>SNKCDVVVVGGGISGMAAAKLLHDSGLNVVVLEARDRVGGRTYTLRNQKVKYVDLGGSYVGPTQNRILRLAKELGLETYKVNEVERLIHHVKGKSYPFRGPFPPVWNPITYLDHNNFWRTMDDMGREIPSDAPWKAPLAEEWDNMTMKELLDKLCWTESAKQLATLFVNLCVTAETHEVSALWFLWYVKQCGGTTRIASTTNGGQERKFVGGSGQVSERIMDLLGDRVKLERPVIYIDQTRENVLVETLNHEMYEAKYVISAIPPTLGMKIHFNPPLPMMRNQMITRVPLGSVIKCIVYYKEPFWRKKDYCGTMIIDGEEAPVAATLDDTKPEGNYAAIMGFILAHKARKLARLTKEERLKKLCELYAKVLGSLEALEPVHYEEKNWCEEQYSGGCYTTYFPPGILTQYGRVLRQPVDRIYFAGTETATHWSGYMEGAVEAGERAAREILHAMGKIPEDEIWQSEPESVDVPAQPITTTFLERHLPSVPGLLRLI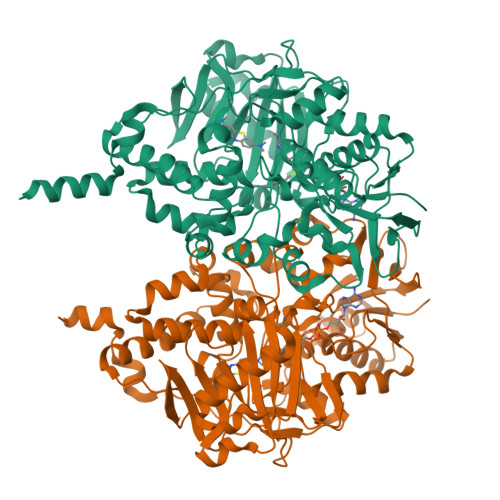GLTTIFSATALGFLAHKRGLLVRV[2x]3-[4-(methylsulfonylamino)phenyl]benzoic acid | C14 H13 N O4 S 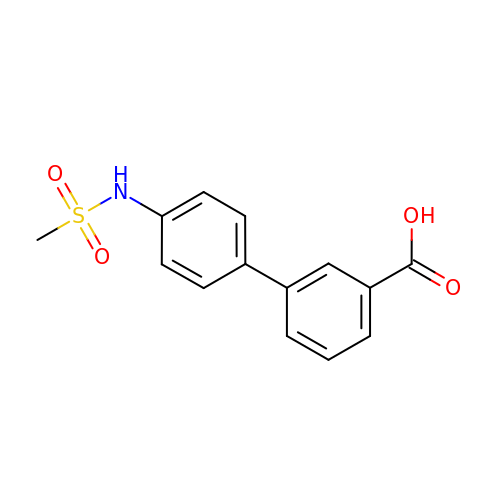| DYJLEZXYMJHNOA-UHFFFAOYSA-N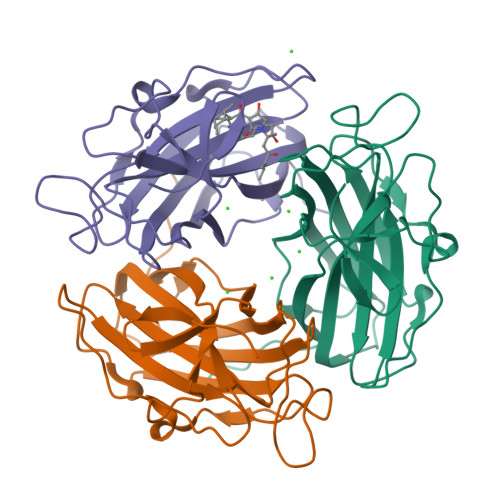>[3x]MTSTVSTDGPVYREYKGFRVNDNIVADFIGVPAVITPGETIEFSVFYTNRGRYAYPDTGLNLVIWFSDRDDLRREDFKLFYKVSRADWQEQDPAKCWDPQFPAEGGVHIACQLSGPDGGILSKPDGTVPLPEVESVTAHVRLAFREGITSEHAGIFALPGMLDAPGDKSIIPGLFGNVFGRLQQASFRLGEGPSSLY> RDFNNLTKGLCTINSWHIYGKDNAVRIGEDSDVLVTREPYVSCDPDECRFYALSQGTTIRGKHSNGTIHDRSQYRALISWPLSSPPTVYNSRVECIGWSSTSCHDGKTRMSICISGPNNNASAVIWYNRRPVTEINTWARNILRTQESECV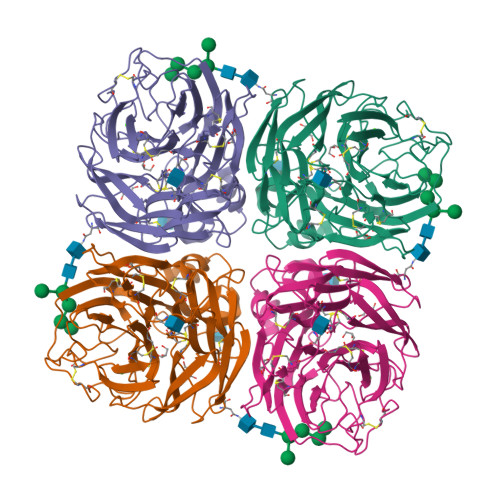CHNGVCPVVFTDGSATGPAETRIYYFKEGKILKWEPLAGTAKHIEECSCYGERAEITCTCRDNWQGSNRPVIRIDPVAMTHTSQYICSPVLTDNPRPNDPTVGKCNDPYPGNNNNGVKGFSYLDGVNTWLGRTISIASRSGYEMLKVPNALTDDKSKPTQGQTIVLNTDWSGYSGSFMDYWAEGECYRACFYVELIRGRPKEDKVWWTSNSIVSMCSSTEFLGQWDWPDGAKIEYFL>[2x]MAHHHHHHSAALEVLFQGPERPLEYEKDDILPMELQNLLPRLEATVTDLKLAHKLDVVKIRQQLQWIHDTIIIIQSTLANGLFPSDFKEYQEMHKYMNAILERKVELFKFINCINEVEPVLSHILDLLEEDLSATPKGNVDFDLLFDLIENCTHESNFLTPNLKQLKECIDAAMEFNEISRDHMDTLDDLINKNVEKCFEIQELKFSSPVRHTPNFTLDQLI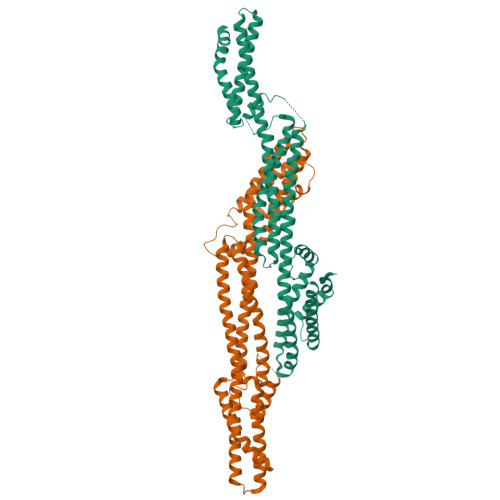KLLSSNNNTTDTMEPKIPNFSPVEESLSRKFLILKRNIPPIEQSLTEILPQRIEQFCGRNIININLLADFLQLKYKRIMKNFRFMMNEIKDLKIELIDKRWNILFINLNNELEYIIEEVRLLLKKINENDDLAQTIKDRFNSQLAKKSKIITKTFNIIYRALEFSLLDAGIALKTNELAKVWVDLRPKSDEILLHIKKFDQSNSSR> MSLTAYMDHKNLANEVIDDARAREITDGVHRVLDRIAAAEEQAGREAGSVRLLAATKTRDIGEIMAAIDAGVRMIGENRPQEVTAKAEGLARRCAERGFSLGVAGAAPDAAAEHIPFHLIGQLQSNKIGKVLPVVDTIESVDSIDLAEKISRRAVARGITVGV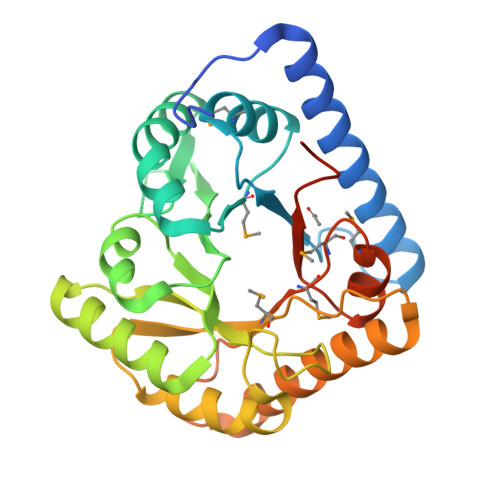LLEVNESGEESKSGCDPAHAIRIAQKIGTLDGIELQGLMTIGAHVHDETVIRRGFSHLRKTRDLILASGEPGTDRCRELSMGMTGDMELAIAEGSTIVRVGTAIFGERAFIEGHHHHHH> FSEQTIPPSAKYGGRHTVTMIPGDGIGPELMLHVKSVFRHACVPVDFEEVHVSSNADEEDIRNAIMAIRRNRVALKGNIETNHNLPPSHKSRNNILRTSLDLYANVIHCKSLPGVVTRHKDIDILIVRENTEGEYSSLEHESVAGVVESLKIITKAKSLRIAEYAFKLAQESGRKKVTAVHKANIMKLGDGLFLQCCREVAARYPQI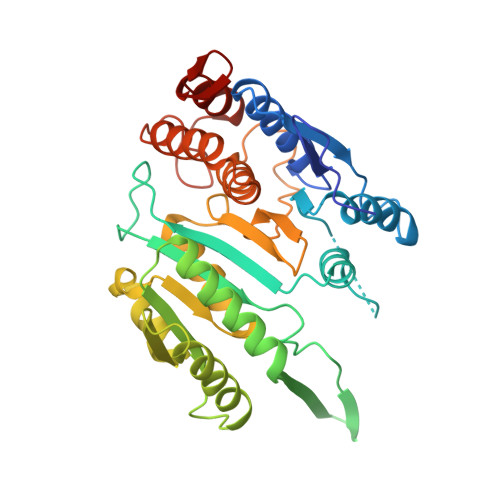TFENMIVDNTTMQLVSRPQQFDVMVMPNLYGNIVNNVCAGLVGGPGLVAGANYGHVYAVFETATRNTGKSIANKNIANPTATLLASCMMLDHLKLHSYATSIRKAVLASMDNENMHTPDIGGQGTTSEAIQDVIRHIRVINGRAVEA> MSFDRPEIYSAPVLQGESPNDDDNTEIIKSFKNFILEFRLDSQFIYRDQLRNNILVKNYSLTVNMEHLIGYNEDIYKKLSDEPSDIIPLFETAITQVAKRISILSRAQSANNNDKDPENTSMDTDSLLLNSLPTFQLILNSNANQIPLRDLDSEHVSKIVRLSGIIISTSVLSSRATYLSIMCRNCRHTTSITINNFNSITGNTVSLPRSCLSTIESESSMANESNIGDESTKKNCGPDPYIIIHESSKFIDQQFLKLQEIPELVPVGEMPRNLTMTCDRYLTNKVIPGTRVTIVGIYSIYNSKNGAGSGRSGGGNGGSGVAIRTPYIKILGIQSDVETSSIWNSVTMFTEEEEEEFLQLSRNPKLYEILTNSIAPSIFGNEDIKKAIVCLLMGGSKKILPDGMRLRGDINVLLLGDPGTAKSQLLKFVEKVSPIAVYTSGKGSSAAGLTASVQRDPMTREFYLEGGAMVL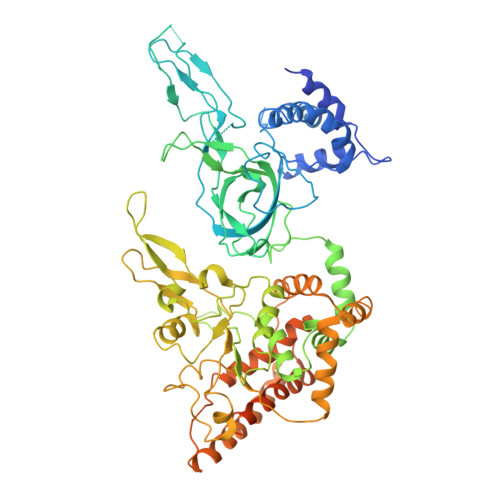ADGGVVCIDEFDKMRDEDRVAIHEAMEQQTISIAKAGITTVLNSRTSVLAAANPIYGRYDDLKSPGDNIDFQTTILSRFDMIFIVKDDHNEERDISIANHVINIHTGNANAMQNQQEENGSEISIEKMKRYITYCRLKCAPRLSPQAAEKLSSNFVTIRKQLLINELESTERSSIPITIRQLEAIIRITESLAKLELSPIAQERHVDEAIRLFQASTMDAASQDPIGGLNQASGTSLSEIRRFEQELKRRLPIGWSTSYQTLRREFVDTHRFSQLALDKALYALEKHETIQLRHQGQNIYRSGV> SPQPLEQIKLSESQLSGRVGMIEMDLASGRTLTAWRADERFPMMSTFKVVLCGAVLARVDAGDEQLERKIHYRQQDLVDYSPVSEKHLADGMT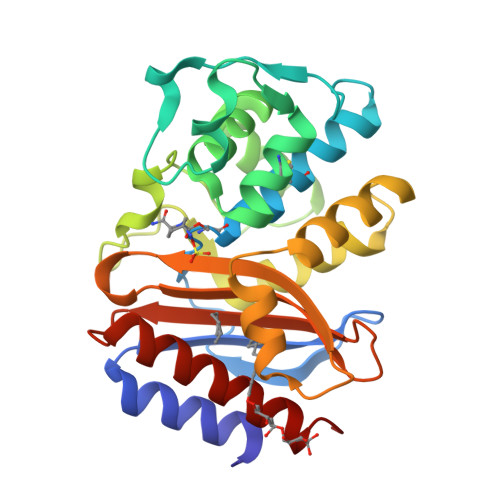VGELCAAAITMSDNSAANLLLATVGGPAGLTAFLRQIGDNVTRLDRWETELNEALPGDARDTTTPASMAATLRKLLTSQRLSARSQRQLLQWMVDDRVAGPLIRSVLPAGWFIADKTGAGERGARGIVALLGPNNKAERIVVIYLRDTPASMAERNQQIAGIGAALIEHWQR>[12x]MEGVGLRAVGSHCSLSEMDDLDLTRALDKPRLKIERKRSFDERSMSELSTGYSRHDGIHDSPRGRSVLDTPLSSARNSFEPHPMMAEAWEALRRSMVFFRGQPVGTLAAVDNTTDEVLNYDQVFVRDFVPSALAFLMNGEPDIVKHFLLKTLQLQGWEKRVDRFKLGEGVMPASFKVLHDPIRETDNIVADFGESAIGRVAPVDSGFWWIILLRAYTKSTGDLTLSETPECQKGMKLILSLCLAEGFDTFPTLLCADGCSMIDRRMGVYGYPIEIQALFFMALRSALSMLKPDGDGREVIERIVKRLHALSFHMRNYFWLDHQNLNDIYRFKTEEYSHTAVNKFNVMPDSIPEWVFDFMPLRGGYFVGNVGPAHMDFRWFALGNCVSILSSLATPDQSMAIMDLLEHRWAELVGEMPLKICYPCLEGHEWRIVTGCDPKNTRWSYHNGGSWPVLLWQLTAACIKTGRPQIARRAVDLIESRLHRDCWPEYYDGKLGRYVGK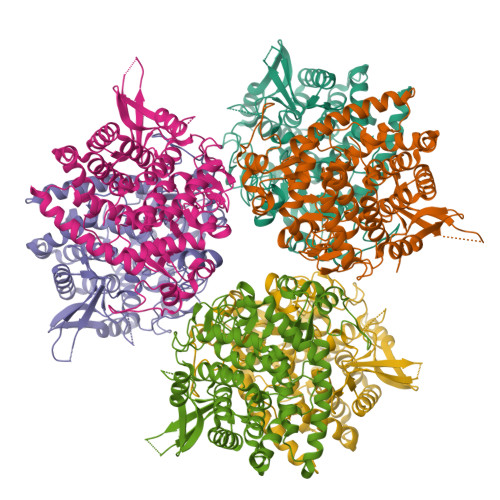QARKYQTWSIAGYLVAKMLLEDPSHIGMISLEEDKLMKPVIKRSASWPQL> KDFLNPKYTLENFIVGEGNRLAYEVVKEALENLGSLYNPIFIYGSVGTGKTHLLQAAGNEAKKRGYRVIYSSADDFAQAMVEHLKKGTINEFRNMYKSVDLLLLDDVQFLSGKERTQIEFFHIFNTLYLLEKQIILASDRHPQKLDGVSDRLVSRFEGGILVEIELDNKTRFKIIKEKLKEFNLELRKEVIDYLLENTKNVREIEGKIKLIKLKGFEGLERKERKERDKLMQIVEFVANYYAVKVEDILSDKRNKRT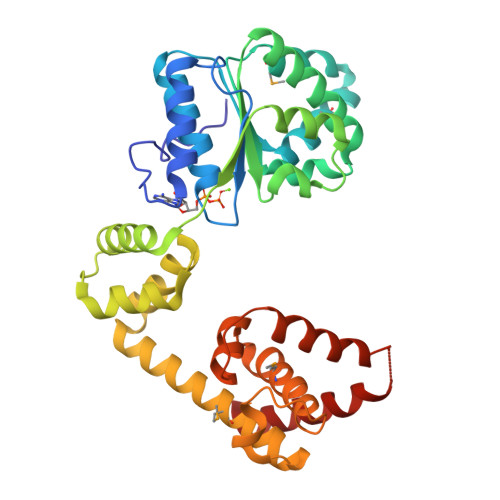SEARKIAMYLCRKVCSASLIEIARAFKRKDHTTVIHAIRSVEEEKKKDRKFKHLVGFLEKQAFDKIC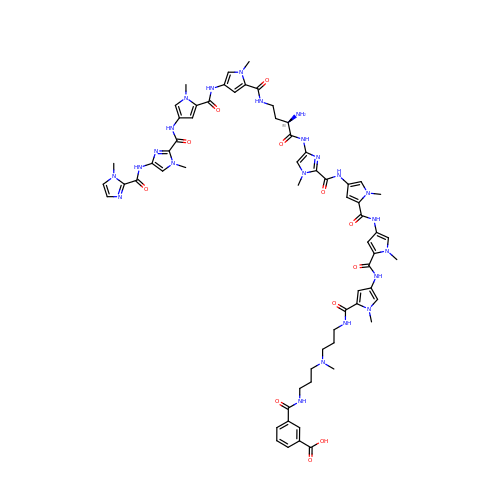3-({3-[(3-{[4-({4-[(4-{[4-({(2R)-2-amino-4-[(1-methyl-4-{[1-methyl-4-({1-methyl-4-[(1-methyl-1H-imidazole-2-carbonyl)amino]-1H-imidazole-2-carbonyl}amino)-1H-pyrrole-2-carbonyl]amino}-1H-pyrrole-2-carbonyl)amino]butanoyl}amino)-1-methyl-1H-imidazole-2-carbonyl]amino}-1-methyl-1H-pyrrole-2-carbonyl)amino]-1-methyl-1H-pyrrole-2-carbonyl}amino)-1-methyl-1H-pyrrole-2-carbonyl]amino}propyl)(methyl)amino]propyl}carbamoyl)benzoic acid | C64 H75 N23 O12 | WKPGYYXGKHNOLO-VZUYHUTRSA-N>[2x]ACGLVASNLNLKPGECLRVRGEVAPDAKSFVLNLGKDSNNLCLHFNPRFNAHGDANTIVCNSKDGGAW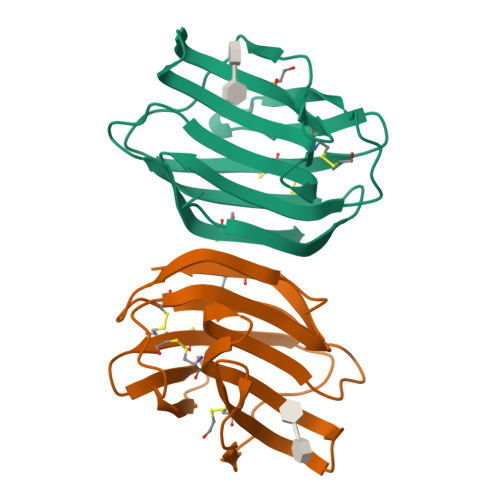GTEQREAVFPFQPGSVAEVCITFDQANLTVKLPDGYEFKFPNRLNLEAINYMAADGDFKIKCVAFD>[4x]MVSDYVPDAGHLVWLNFTPQA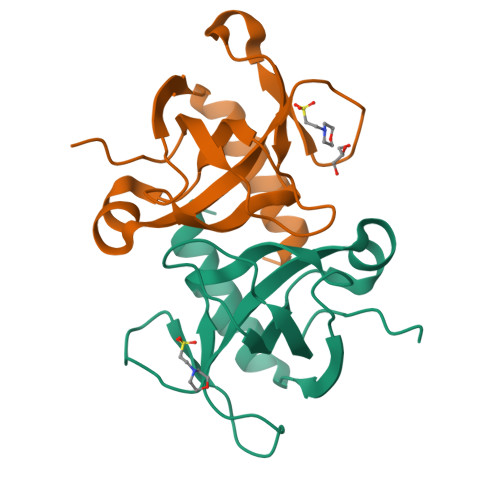GHEQGGRRPALVLSPAAYNGVTGLMQACPVTSRAKGYPFEVTLPAHLGVSGVVLADHCRSLDWRSRRAEQLAEAPADVLAEVRGKLGSLLGMSEKA6-{[(3R,4R)-4-(2-{[(1R,2S)-2-(3-chlorophenyl)cyclopropyl]amino}ethoxy)pyrrolidin-3-yl]methyl}-4-methylpyridin-2-amine 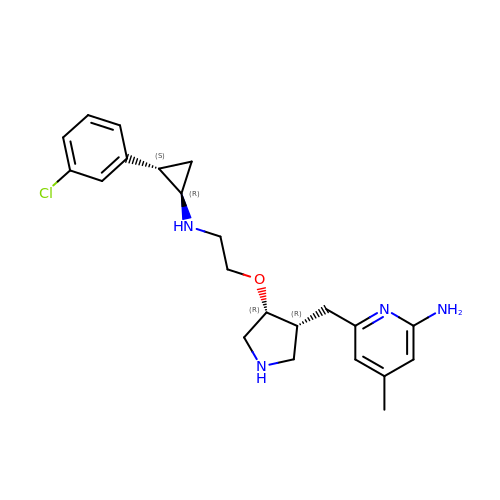| C22 H29 Cl N4 O | SLFXGXAWJWFFCO-RCOXNQKVSA-N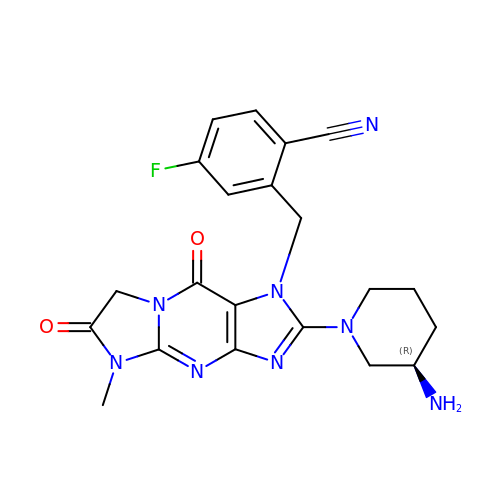2-({2-[(3R)-3-aminopiperidin-1-yl]-5-methyl-6,9-dioxo-5,6,7,9-tetrahydro-1H-imidazo[1,2-a]purin-1-yl}methyl)-4-fluorobenzonitrile | C21 H21 F N8 O2 | KMOYVYIQCXEQDG-OAHLLOKOSA-N> MAKVRIYQLAKELGMETQELLELLDQMGVAYKSHASTLEEKDAEAVRELVKEQRGLQEKLAEEERRKSLPRRPPVVVIMGHVDHGKTTLLDYLRKSRIAEKEAGGITQHVGAFEVKTPQGTVVFIDTPGHEAFTTIRQRGAKVADIAVIVIAADDGIMPQTEEAIAHAKAAGAKLIFAINKIDLPQADPEKVKRQLMERGFVPEEYGGDAIVIPISAKTGQGVQDLLEMILLLAELEDYRADPNAEPRGVILESKLDKQAGIIANMLVQEGTFRVGDYVVAGEAYGRIRAMMDADGNQRKEAGPGSAVQVLGFQELPHAGDVVEWVPD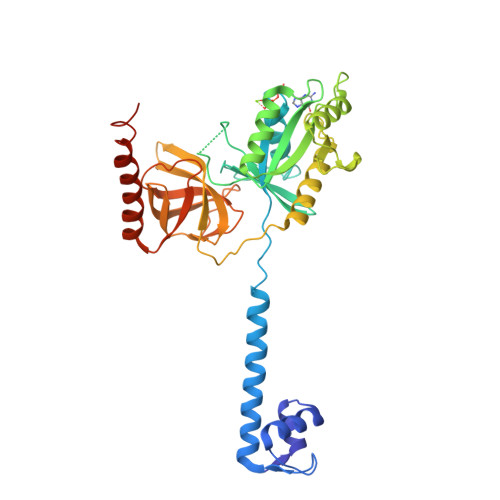LEAAKEIAEERKEERKAREEEEKARRPRTMAELLR>XMEAAHSKSTEECLAYFGVSETTGLTPDQVKRHLEKYGHNELPAEEGKSLWELVIEQFEDLLVRILLLAACISFVLAWFEEGEETITAFVEPFVILLILIANAIVGVWQERNAENAIEALKEYEPEMGKVYRADRKSVQRIKARDIVPGDIVEVAVGDKVPADIRILSIKSTTLRVDQSILTGESVSVIKHTEPVPDPRAVNQDKKNMLFSGTNIAAGKALGIVATTGVSTEIGKIRDQMAATEQDKTPLQQKLDEFGEQLSKVISLICVAVWLINIGHFNDPVHGGSWIRGAIYYFKIAVALAVAAIPEGLPAVITTCLALGTRRMAKKNAIVRSLPSVETLGCTSVICSDKTGTLTTNQMSVCKMFIIDKVDGDFCSLNEFSITGSTYAPEGEVLKNDKPIRSGQFDGLVELATICALCNDSSLDFNETKGVYEKVGEATETALTTLVEKMNVFNTEVRNLSKVERANACNSVIRQLMKKEFTLEFSRDRKSMSVYCSPAKSSRAAVGNKMFVKGAPEGVIDRCNYVRVGTTRVPMTGPVKEKILSVIKEWGTGRDTLRCLALATRDTPPKREEMVLDDSSRFMEYETDLTFVGVVGMLDPPRKEVMGSIQLCRDAGIRVIMITGDNKGTAIAICRRIGIFGENEEVADRAYTGREFDDLPLAEQREACRRACCFARVEPSHKSKI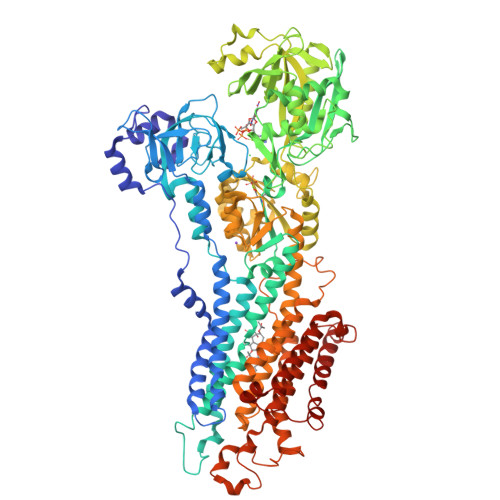VEYLQSYDEITAMTGDGVNDAPALKKAEIGIAMGSGTAVAKTASEMVLADDNFSTIVAAVEEGRAIYNNMKQFIRYLISSNVGEVVCIFLTAALGLPEALIPVQLLWVNLVTDGLPATALGFNPPDLDIMDRPPRSPKEPLISGWLFFRYMAIGGYVGAATVGAAAWWFMYAEDGPGVTYHQLTHFMQCTEDHPHFEGLDCEIFEAPEPMTMALSVLVTIEMCNALNSLSENQSLMRMPPWVNIWLLGSICLSMSLHFLILYVDPLPMIFKLKALDLTQWLMVLKISLPVIGLDEILKFIARNYLEG[2x]>[2x]MKNYSFYQFVMTVRGRHDDKGRLAEE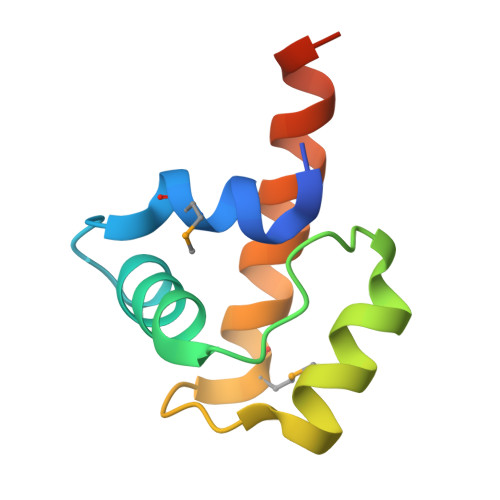IFDDLAFPKHDDDFNILSDYIETHGDFTLPMSVFDDLYEEYTEWLKFLEHHHHHH> LFQTSYTLENQGSVICIPNNGQCFCLAWLKSNGTNAEKLAANILQWISFALSALCLMFYGYQTWKSTCGWENIY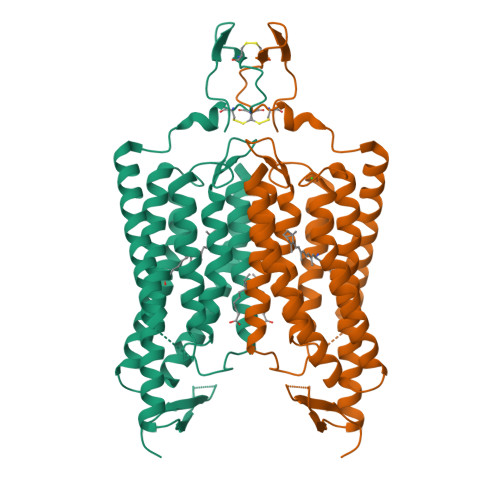VATIQMIKFIIEYFHSFDEPAVIYSSNGNKTRWLRYASWLLTCPVILIHLSNLTGLANDYNKRTMGLLVSDIGTIVWGTTAALSKGYVRVIFFLMGLCYGIYTFFNAAKVYIEAYHTVPKGRCRQVVTGMAWLFFVSWGMFPILFILGPEGFGVLSRYGSNVGHTIIDLMSKQCWGLLGHYLRVLIHSHILIHGDIRKTTKLNIGGTEIEVETLVEDE>[2x]MALSLCVLFTLASVVSGHVAHPSLGRGDGFPFLWDNAASTLDQLNGTDTTIILNGFNYLDRLSMFKTVLEGTRKYFDSFAPNNTANIYWGFTIYLNWILATGRSADP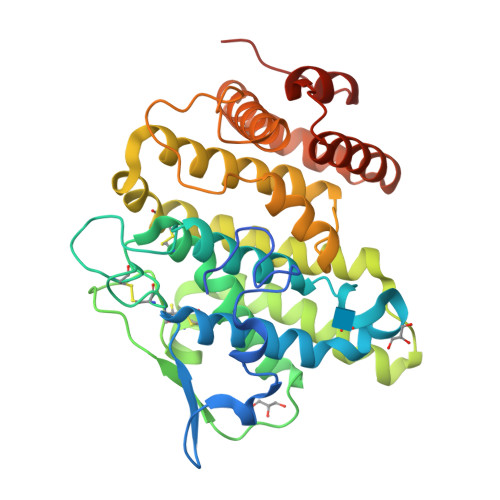TGHTTCGLAHGDPMCLAEESWWNCIKYNPAAIAFFAAKKAGIFGDVTKTIVLAKPKEANSPYCSSEEECQAAYPDVMATYLDYFEYLMSLEKTGESIDMDKAQQLLWKAHVTSMENSIAVCKPRLKNYNIIERQLDRDYLISLLYFAATNFPTNFIESIKFVADMPHRQLRFGDIAPFIPDMDMKKNNLLVVLHGFYTVHSLSGGSSLTHWRNLMESPVSREMARDMVNLILAGTPVEVQVELAKLGIPTPVDYKDDDK>SLKSTDDLNKCIDHISVLIKDAYLLYTNESFATSTFISITIIEEVGKTHIGMFISENKDIKRGKDPLRNHKSKHAFGSLPTIKMGGRLNKAIGDEMIDKIVEDAETGELISIRESSLYADIIDDILEVPSEKISKEQ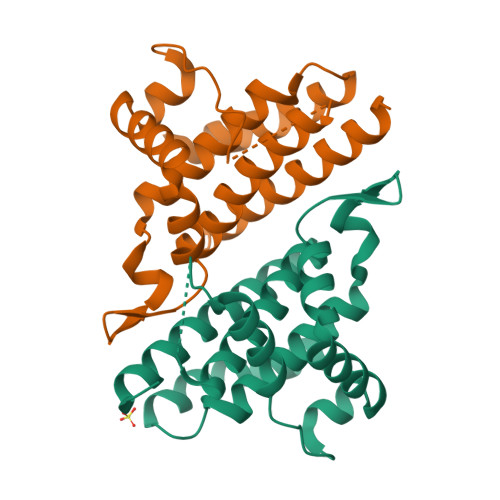SRALLLYAIECFDDSLVGYTHHSFEVSETTDELFEKLANNKHHHHHH[24x]>[2x]GPSSVIARVALAHEDDVGKNIVR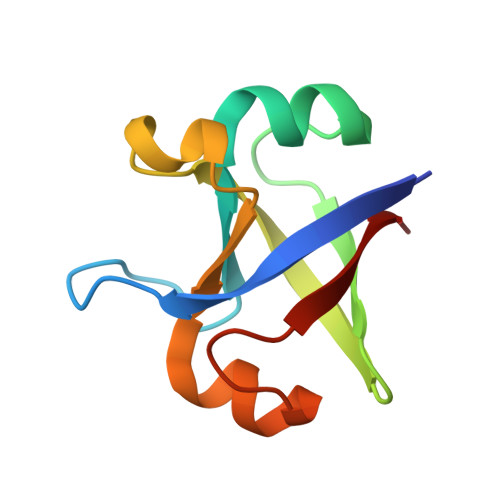MDEELMRLLGVKVGDLVEIMKVSSVIARVALAHEDDVGKNIVRMDEELMRLLGVKVGDLVEIMKV> MKSADDVKKVFHILDKDKSGF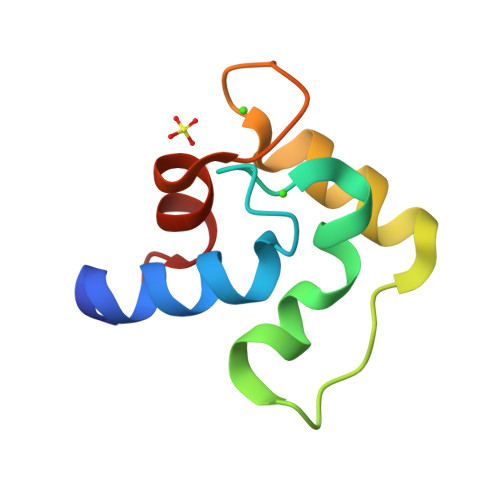IEEDELGSILKGFSSDARDLSAKETKTLMAAGDKDGDGKIGVEEFSTLVAES>[4x]HPPPTDSTLRPMFKRLLANAECQEGQSVCFEIRVSGIPPPTLKWEKDGQPLSLGPNIEIIHEGLDYYALHIRDTLPEDTGYYRVTATNTAGSTSCQAHLQVERLR

Titin has a molecular weight of more than 3 MDa in its longest isoform and is over 1.5 μm in length, spanning half of a sarcomeric unit from the peripheral Z-disk to the central M-band[3–5]. Taking titin kinase as the N-terminal boundary of the titin M-band segment, there are another ten Ig domains towards the far C-terminus of titin, referred to as M1 to M10, encoded by at least six exons 358–363, or Mex1 to Mex6, on the respective TTN gene. To achieve this goal, we have solved the crystal structures of five titin M-band domains: M1, M3, M4, M7, and M10. In addition to the ABDE/A’CC’FG β-sheet sandwich core, all M-band domain structures comprise two characteristic tip regions, which we refer to as “N-tip” and “C-tip” due to their proximity to the N-termini and C-termini of the respective domains.

The second segment in the pairwise analysis of spatial deviations ranges from the A’B loop to the DE loop. This region features several significant individual M-band domain deviations for M1 (BC loop), M3 (C’D loop, DE loop), and M7 (DE loop), indicating potential M-band domain signature motifs (discussed in more detail below). In our analysis of titin M-band domains, the C’D loops of M3 and M10 are flagged for being most diverse. In four of the six structures (M1, M4, M7, M10), D73 (M1), also invariant in all M-band sequences, forms an additional salt bridge with a conserved lysine/arginine (K52 in M1), located at the CD loop that connects two β-strands from the two opposite β-sheets. The conserved lysine/arginine position in the M3 domain is replaced by an asparagine (N52 in M3, K52 in M1), and hence no interaction with the equivalent aspartate (D74 in M3, D73 in M1) is found. As N52 in M3 is close to an M3 structural motif that significantly deviates from the other structures, it is plausible that the loss of this specific interaction is of functional relevance and part of a specific M3 signature. By contrast, the three cysteines of the M3 domain (C18, C25, C91, equivalent to G17, K24, S90 in M1), which are located in different β-strands A’, B, and G, are all at least partially surface exposed. As expected, we found one free cysteine equivalent for domains M4 and M10, and almost three free cysteine equivalents for M3. Unlike our findings for M4 and M10, size exclusion chromatography of the M3 domain under non-reducing conditions revealed a mixture of different higher molecular weight species. We attribute this to possible combinatorial linkages through all three exposed cysteine residues under the given experimental conditions. In the corresponding SDS-PAGE analysis, higher molecular weight species were only faintly detectable.> AKCVSYGVAQIKA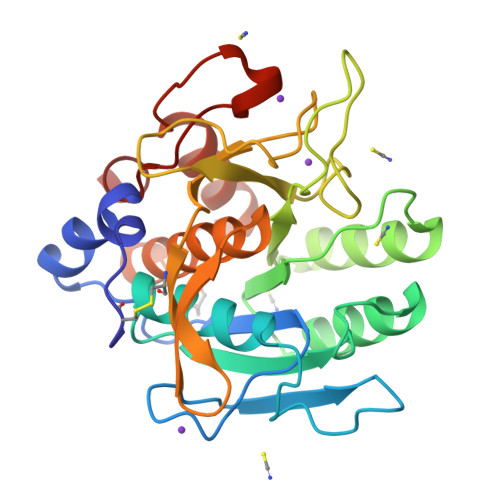PALHSQGYTGSNVKVAILDTGIDSSHPDLNVAGGASFVPSETNPFQDNSSGGTHIAGTVLAVAPSASLYAVKVLGADGKGQASWIINGIEWAIANNMDVINMSLGSPSGSAAVKAAVDKAVASGVVVVAAAGNSGTSGSSSTVTYPAKYPSVIAVGAVDSSNQRAPFSSVGPELDVMAPGVSICSTLPGGKYGALSGTSMASPHVAGAAALILSKHPNWTNTQVRSSLENTATKLGDSFYYGKGLINVEAAAQ>MSEEQSHADQDAYVADVDGILDVLRAQVLERKPDDIFQFISKSALSLQKDRGAESCDRINCKVKDEQKSRALTIIVFGASGDLAKKKTFPALFDLYCGGLLPPEVNIIGYARTKVDDVEKWKHETLMKYFSNLSERGCHAEDFLKHISYFCGAYDSVDDFKRLDAVIREKENAFKGPEKGGNRLFYLALPPSVFASVCESIHKGAMPQEVGGWVRVIIEKPFGRDTKSSAELSQALEPFFDESQLYRIDHYLGKEMVQNIITTRFANRIFSAVWNASNIACVQITFKETIGTEGRGGYFDNIGIIRDVMQNHLTQILALLAMEKPRSLDAECIRDEKVSVLKCIEPITKENCVLGQYTASADGSIPGYLEDVTVPEGSTCPTFAVMRLNINNDRWAGVPFILKAGKAVEQKYVA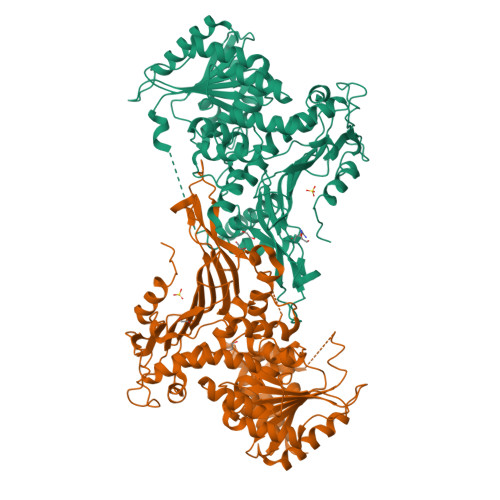IRIQFRDEVHPYGEATQRNELVIRAQPSEAMYVKITTKVPGLSGDLRQTHQTELDLTYHTRYDVRLPDAYESLINDALLGNSTNFVRKDELDVAWRIFTPLLHQIDSGEIKPIPYQAGTRGPKEADEFIANNGFKHQKGYHWLPSNKL[4x]> GS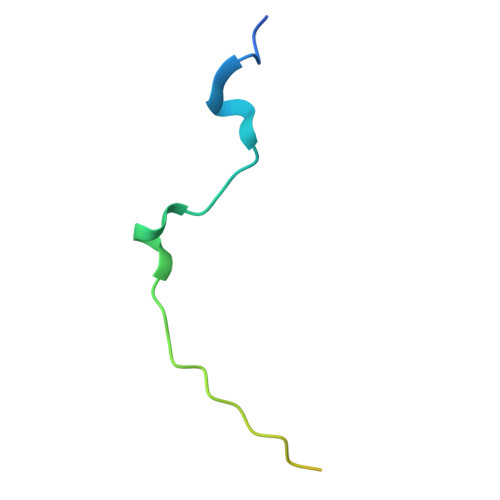KTLMGNPWFQRKKLPSVLLFKKPSPFIFISQRPSPETQDTIHPLDEEAFLK> MVNFDLGQVGEVFRRKDKGAIVSGDNPEEEEDVDASEFEEDEVKPVRTKNRRPKEDAFTQQRLAAINPVLTPRTVLPLYLLIAVVFVIVGGCILAQNSKVDEVTIYYQDCMTNATSSWSDIPSEHWQFVFHKYKTY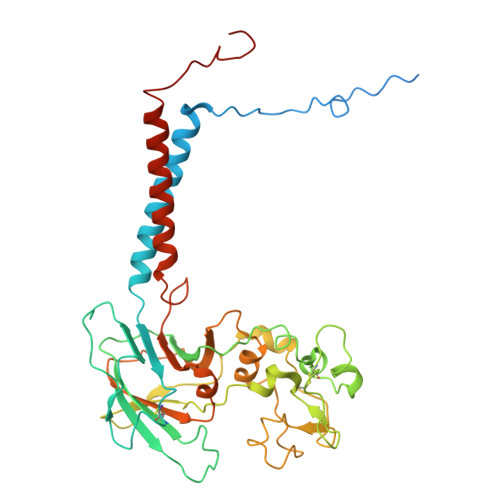NTAPQWRFVDDESDDFTKQRGTCQIRFTTPSDMKNNVYLNYVLEKFAANHRRYVLSFSEDQIRGEDASYETVHDATGINCKPLSKNADGKIYYPCGLIANSMFNDTFPLQLTNVGDTSNNYSLTNKGINWESDKKRYKKTKYNYTQIAPPPYWEKMYPDGYNETNIPDIQDWEEFQNWMRPGAFDKITKLIRINKNDTLPAGEYQLDIGLHWPVLEFNGKKGIYLTHGSHLGGRNPFLGIVYLIGGCICAAMALILLTFWLFGGRKIADASSLSWNMK> MHKRFLGTIFGATLTCFQAQAAQFQCQDDVKPTSYTTEEQKLVDQFWNESLIYLDQYLKALETPTGQCKDSAQAT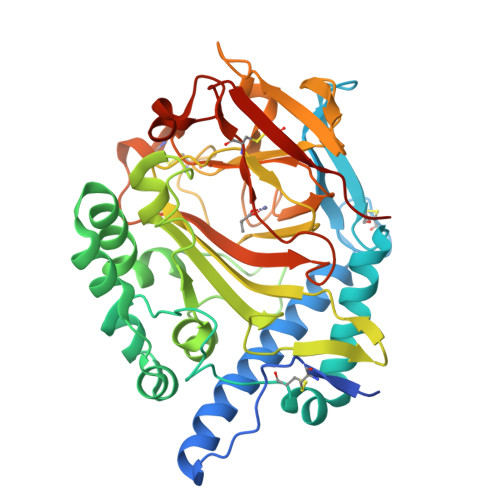IQTYNSETGKMQTQCIMKYRDVELVAKHLKAVLAEPDKAKACFDPQKNYKAFPLYTPSAHVQNLSATSKWINRPLLTDYYKKIGGEIGAAGLELNENFLEITSRTDTTLHWTKDVSIKGLPTLWSSVGWIPFYAENPNAGSDRFRGGYLYAEVMGPWGNLRIKEIDGEKVGAEIGMTAQLFNTSAPYHYHHPQEIYMTLTKPQCIDQNKHMVMHWDNNQFKQKRSDNGWTVNIDGSKGKWKKWFSNQDPEQNWLTYFERNAIHAFHTLEGCNQTIKNSGLVTVWARTTAQDNNQTTQLCRPMTGAKDIKTMKPEDKAICDLDDWKPHHHHHH> GMFVWHEYENAAEAAQSLADAVADALQGALDEKGGAVLAVSGGRSPIAFFNALSQKDLDWKNVGITLADERIVPTNHADSNTGLVREYLLKNKAAAAVWIPM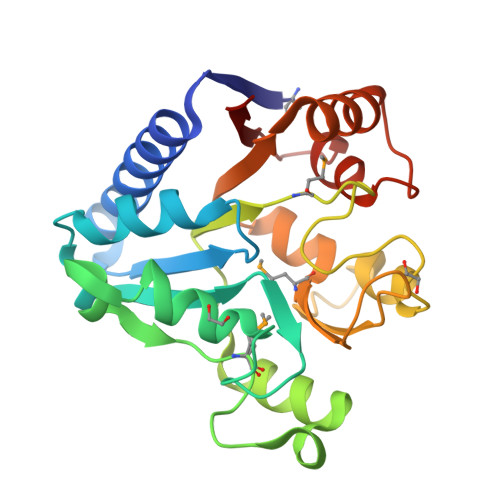VEDGKTETELHPDAVVDYALKHYKQPDVLILGMGNDGHTASIFPKAPQFQTAIDGSAGVALVHTTPVTAPHERISMTLDAIAHTGHVFLAIQGEEKKAVFDQAAQGENREYPISLVLNHQGVNCHVFYAE>[4x]GMDDQSGDQ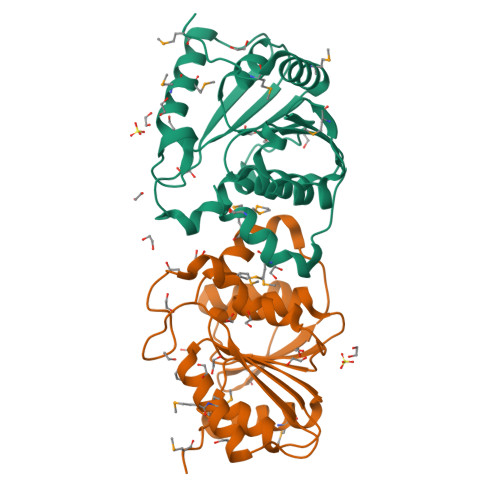MRPELTMPPAEAEALRMAYEEAEVILEYGSGGSTVVAAELPGKHVTSVESDRAWARMMKAWLAANPPAEGTEVNIVWTDIGPTGDWGHPVSDAKWRSYPDYPLAVWRTEGFRHPDVVLVDGRFRVGCALATAFSITRPVTLLFDDYSQRRWQHQVEEFLGAPLMIGRLAAFQVEPQPIPPGSLMQLIRTMTSP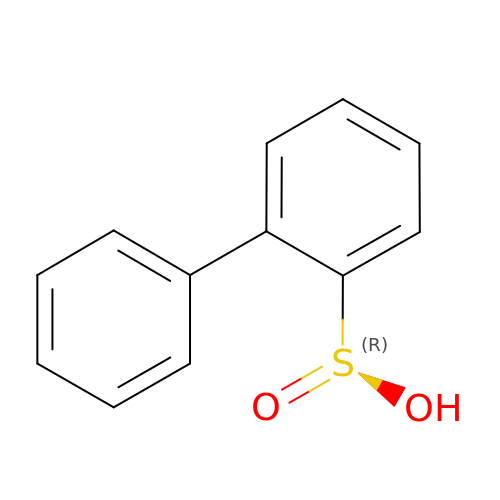1,1'-BIPHENYL-2-SULFINIC ACID | C12 H10 O2 S | LZCLZDCSBDVAOV-UHFFFAOYSA-N>GSHMSAPLPLDELRTFAEVLDRVKAAYVEPVDDKTLLENAIKGMLSNLDPHSAYLGPEDFAELQESTSGEFGGLGIEVGSEDGFIKVVSPIDDTPAARAGIQPGDLIVQIDGKPTKGQSMTEAVDSMRGKAGSPITLTIVRDGGRPFDVELKRAIIKVKSVKSQVLEPGYAYLRITQFQVNTGEEVVKALNQLRKDNKGRLKGLVLDLRNNPGGVLQSAVEVADAFLTKGLIVYTKGRIANSELRFSADPADPSDKVPLVVLINGGSAAAAEIVAGALQDQKRAILMGTDSFGKGSVQTVLPLNNDRALKLTTALYYTPNGRSIQAQGIVPDIEVGRAKVTQERSSFEGFKEADLQGHLANGNGGADRPTGKRAAPSERPQDSDYQLSQALSLLKGLSVTRGN[3x];> MEDTAVETKAKPEKYGSFSEDSLYSLLVAELAGQRNRFDIALSNYVVQAQKTRDPGVSERAFRIAEYLGADQEALDTSLLWARSAPDNLDAQRAAAIQLARAGRYEESMVYMEKVLNGQGDTHFDFLALSAAETDPDTRAGLLQSFDHLLKKYPNNGQLLFGKALLLQQDGRPDEALTLLEDNSASRHEVAPLLLRSRLLQSMKRSDEALPLLKAGIKEHPDDKRVRLAYARLLVEQNRLDDAKAEFAGLVQQFPDDDDLRFSLALVCLEAQAWDEARIYLEELVERDSHVDAAHFNLGRLAEEQKDTARALDEYAQVGPGNDFLPAQLRQTDVLLKAGRVDEAAQRLDKARSEQPDYAIQLYLIEAEALSNNDQQEKAWQAIQEGLKQYPEDLNLLYTRSMLAEKRNDLAQMEKDLRFVIAREPDNAMALNALGYTLADRTTRYGEARELILKAH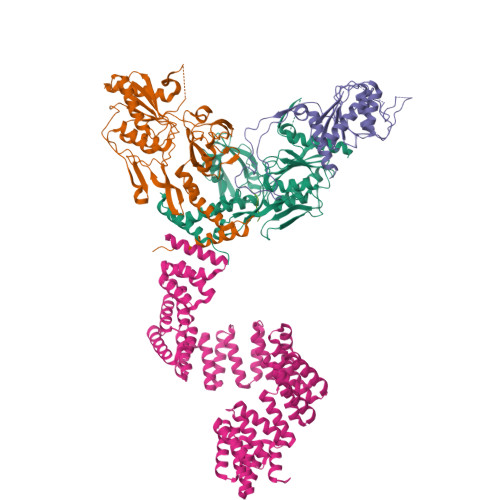KLNPDDPAILDSMGWINYRQGKLADAERYLRQALQRYPDHEVAAHLGEVLWAQGRQGDARAIWREYLDKQPDSDVLRRTIKRLTGAETP> PDSVDYRKKGYVTPVKNQGQCGSCWAFSSVGALEGQLKKKTGKLLNLSPQNLVDCVSENDGCGGGYMTNAFQYVQKNRGIDSEDAYPYVGQEESCMYNPTGKAAKCRGYREIPEGNEKALKRAVARVGPVSVAIDASLTS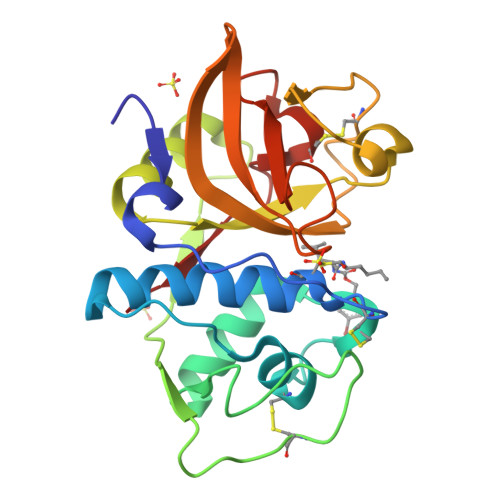FQFYSKGVYYDESCNSDNLNHAVLAVGYGIQKGNKHWIIKNSWGENWGNKGYILMARNKNNACGIANLASFPKM>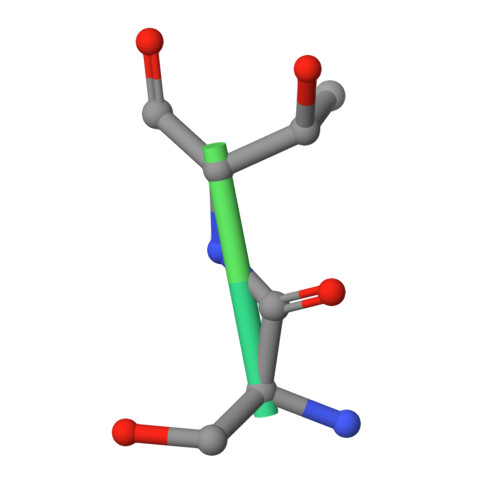 FPTSTSLSPFYLR>[6x]APTKRKGECPGAAPKKPKEPVQVPKLLIKGGVEVLEVKTGVDAITEVECFLNPEMGDPDENLRGFSLKLSAENDFSSDSPERKMLPCYSTARIPLPNLNEDLTCGNLLMWEAVTVQTEVIGITSMLNLHAGSQKVHEHGGGKPIQGSNFHFFAVGGDPLEMQGVLMNYRTKYPDGTITPKNPTAQSQVMNTDHKAYLDKNNAYPVECWVPDPSRNENTRYFGTFTGGENVPPVLHVTNTATTVLLDEQGVGPLCKADSLYVSAADICGLFTNSSGTQQWRGLARYFKIRLRKRSVKN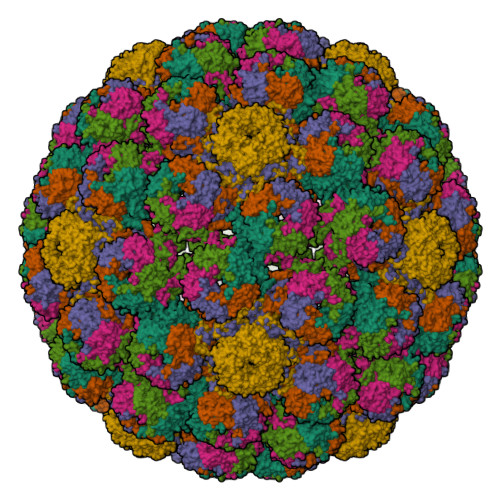PYPISFLLSDLINRRTQRVDGQPMYGMESQVEEVRVFDGTERLPGDPDMIRYIDKQGQLQTKML;> GAALALLGDLVASVSEAAAATGFSVAEIAAGEAAAAIEVQIASLATVEGITSTSEAIAAIGLTPQTYAVIAGAPGAIAGFAALIQTVSGISSLAQVGYRFFSDWDHKVSTVGLYQQSGMALELFNPDEYYDILFPGVNTFVNNIQYLDPRHWGPSLFATISQALWHVIRDDIPSITSQELQRRTERFFRDSLARFLEETTWTIVNAPINFYNYIQQYYSDLSPIRPSMVRQVAEREGTRVHFGHTYSIDDADSIEEVTQRMDLRNQQSVHSGEFIEKTIAPGGANQRTAPQWMLPLLLGLYGTVTPALEAYEDGPNQKKRRVSRGSSQKAKGTRASAKTTNKRRSRSSRS> MHWQTHTVFNQPIPLNNSNLYLSDGALCEAVTREGAGWDSDFLASIGQQLGTAESLELGRLANVNPPELLRYDAQGRRLDDVRFHPAWHLLMQALCTNRVHNLAWEEDARSGAFVARAARFMLHAQVEAGSLCPITMTFAATPLLLQMLPAPFQDWTTPLLSDRYDSHLLPGGQKRGLLIGMGMTEKQGGSDVMSNTTRAERLEDGSYRLVGHKWFFSVPQSDAHLVLAQTAGGLSCFFVPRFLPDGQRNAIRLERLKDKLGNRSNASCEVEFQDAIGWLLGLEGE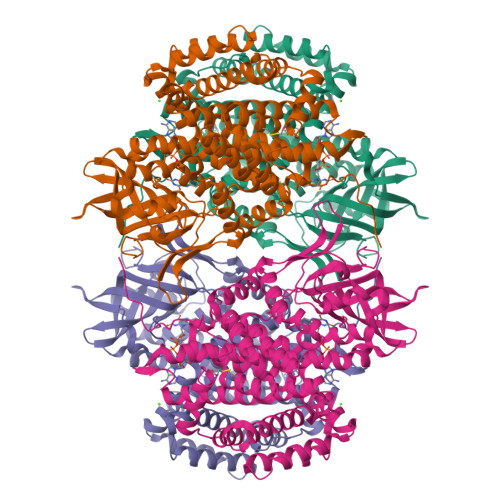GIRLILKMGGMTRFDCALGSHAMMRRAFSLAIYHAHQRHVFGNPLIQQPLMRHVLSRMALQLEGQTALLFRLARAWDRRADAKEALWARLFTPAAKFVICKRGMPFVAEAMEVLGGIGYCEESELPRLYREMPVNSIWEGSGNIMCLDVLRVLNKQAGVYDLLSEAFVEVKGQDRYFDRAVRRLQQQLRKPAEELGREITHQLFLLGCGAQMLKYASPPMAQAWCQVMLDTRGGVRLSEQIQNDLLLRATGGVCV>[6x]ADCAWLEAQEEEEVGFPVRPQVPLRPMTYKAALDISHFLKEKGGLEGLIWSQRRQEILDLWIYHTQGYFPDWQNYTPGPGIRYPLTFGWCFKLVPVEPEKVEEANEG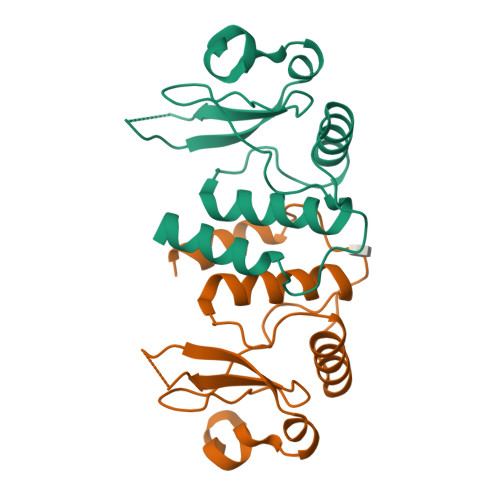ENNSLLHPMSLHGMEDAEKEVLVWRFDSKLAFHHMARELHPEYY> MKKEKIDLFYGAL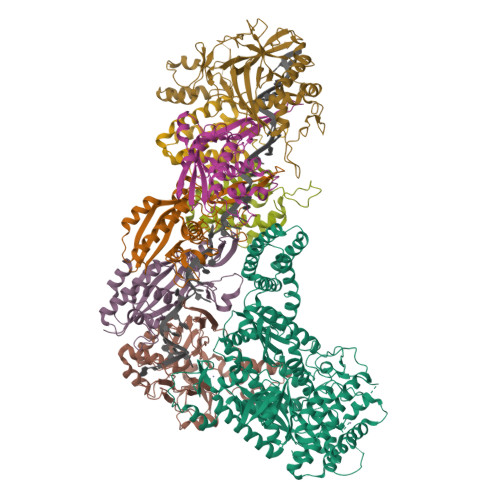LHDIGKVIQRATGERKKHALVGADWFDEIADNQVISDQIRYHMANYQSDKLGNDHLAYITYIADNIASGVDRRQSNEESDEDTSAKIWDTYTNQADIFNVFGAQTDKRYFKPTVLNLKSKPNFASATYEPFSKGDYAAIATRIKNELAEFEFNQVQIDSLLNLFEATLSFVPSSTNTKEIADISLADHSRLTAAFALAIYDYLEDKGRHNYKEDLFTKVSAFYEEEAFLLASFDLSGIQDFIYNINIATNGAAKQLKARSLYLDFMSEYIADSLLDKLGLNRANMLYVGGGHAYFVLANTEKTVETLVQFEKDFNQFLLANFQTRLYVAFGWGSFAAKDIMSELNSPESYRQVYQKASRMISKKKISRYDYQTLMLLNRGGKSSERECEICHSVENLVSYHDQKVCDICRGLYQFSKEIAHDHFIITENEGLPIGPNACLKGVAFEKLSQEAFSRVYVKNDYKAGTVKATHVFVGDYQCDEIYNYAALSKNENGLGIKRLAVVRLDVDDLGAAFMAGFSQQGNGQYSTLSRSATFSRSMSLFFKVYINQFASDKKLSIIYAGGDDVFAIGSWQDIIAFTVELRENFIKWTNGKLTLSAGIGLFADKTPISLMAHQTGELEEAAKGNEKDSISLFSSDYTFKFDRFITNVYDDKLEQIRYFFNHQDERGKNFIYKLIELLRNHDRMNMARLAYYLTRLEELTRETDRDKFKTFKNLFYSWYTNKNDKDRKEAELALLLYIYEIRKD;> MTYKLYIMTFQNAHFGSGTLDSSKLTFSADRIFSALVLEALKMGKLDAFLAEANQDKFTLTDAFPFQFGPFLPKPIGYPKHDQIDQSVDVKEVRRQAKLSKKLQFLALENVDDYLNGELFENEEHAVIDTVTKNQPHKDDNLYQVATTRFSNDTSLYVIANESDLLNELMSSLQYSGLGGKRSSGFGRFELDIQNIPLELSDRLTKNHSDKVMSLTTALPVDADLEEAMEDGHYLLTKSSGFAFSHATNENYRKQDLYKFASGSTFSKTFEGQIVDVRPLDFPHAVLNYAKPLFFKLEV;>[2x]MTILTDENYVDIAEKAILKLERNTRNRKNPDAFFLTTSKLRNLLSLTSTLFDESKVKEYDALLDRIAYLRVQFVYQAGREIAVKDLIEKAQILEALKEIKDRETLQRFCRYMEALVAYFKFYGGKD;>[3x]MTFAKIKFSAQIRLETGLHIGGSDAFAAIGAIDSPVIKDPITNLPIIPGSSLKGKMRTLLAKVYNEKVAEKPSDDSDILSRLFGNSKDKRFKMGRLIFRDAFLSNADELDSLGVRSYTEVKFENTIDRITAEANPRQIERAIRNSTFDFELIYEITDENENQVEEDFKVIRDGLKLLELDYLGGSGSRGYGKVAFENLKATTVFGNYDVKTLNELLTAEV;> MKNDYRTFKLSLLTLAPIHIGNGEKYTSREFIYENKKFYFPDMGKFYNKMVEKRLAEKFEAFLIQTRPNARNNRLISFLNDNRIAERSFGGYSISETGLESDKNPNSAGAINEVNKFIRDAFGNPYIPGSSLKGAIRTILMNTTPKWNNENAVNDFGRFPKENKNLIPWGPKKGKEYDDLFNAIRVSDSKPFDNKSLILVQKWDYSAKTNKAKPLPLYRESISPLTKIEFEITTTTDEAGRLIEELGKRAQAFYKDYKAFFLSEFPDDKIQANLQYPIYLGAGSGAWTKTLFKQADGILQRRYSRMKTKMVKKGVLKLTKAPLKTVKIPSGNHSLVKNHESFYEMGKANFMIKEIDK> MMSREKAAGTFFKDYQKKNVMRLLQDSLEKIINEWLKTDDESHTKLKSLQELSEMDINATS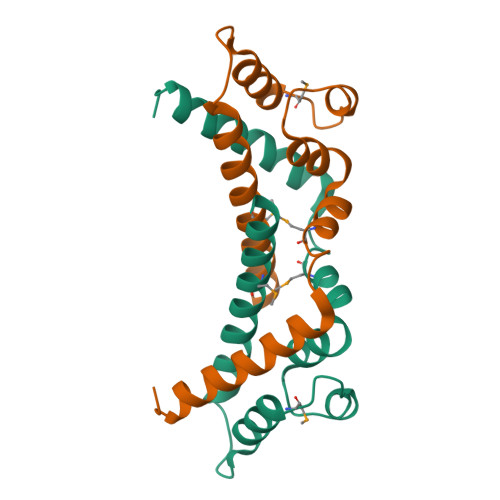FAEHSPLPDFVTRLWLDPHKALDAMDKNISKNEIRKLIKETAREIELVFTHQKAPDYS(E)-4-((2-nicotinoylhydrazono)methyl)benzimidamide 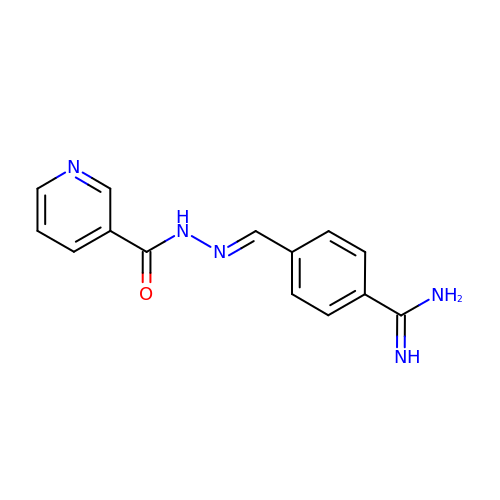| C14 H13 N5 O | DDBLYJHCQJAIJN-QGMBQPNBSA-N>[5x]MGNNLMQTDLSVWGMYQHADIVVKCVMIGLILASVVTWAIFFSKSVEFFNQKRRLKREQQLLAEARSLNQANDIAADFGSKSLSLHLLNEAQNELELSEGSDDNEGIKERTSFRLERRVAAVGRQMGRGNGYLATIGAISPFVGLFGTVWGIMNSFIGIAQTQTTNLAVVAPGIAEALLATAIGLVAAIPAVVIYNVFARQIGGFKAMLGDVAAQVLLLQSRDLDLEASAAAHPVRVAQKLRAG;>[2x]MAMHLNENLDDNGEMHDINVTPFIDVMLVLLIIFMVAAPLATVDVKVNLPASTSTPQPRPEKPVYLSVKADNSMFIGNDPVTDETMITALNALTEGKKDTTIFFRADKTVDYETLMKVMDTLHQAGYLKIGLVGEETAKAKENLYFQGNAGSGHHHHHHHHHH

Ton is a membrane protein complex found in the inner membrane of Gram-negative bacteria. Ton can be described as a molecular motor in which the ExbB and ExbD subunits assemble to form a proton channel and use the proton gradient across the cytoplasmic membrane. The energy derived from proton translocation is propagated through the elongated TonB subunit that spans the periplasmic space and physically interacts with numerous TonB dependent transporters (TBDT) at the outer membrane, allowing the active transport of rare nutrients into the periplasm.

To gain further information on structure and stoichiometry, we performed a single particle cryo-electron microscopy (cryo-EM) analysis on the full-length ExbB–ExbD complex reconstituted in lipid nanodiscs. The final reconstruction used 85,936 particles and yielded a 3.3 Å overall resolution structure calculated without imposing symmetry. As found in the crystal structure, ExbB assembles as a pentamer, but instead of one ExbD TM domain, two TM helices of ExbD are now clearly resolved in the TM pore defined by the ExbB pentamer. The two TM helices are parallel but shifted relative to one another by half a helical turn. The two essential aspartate residues at position 25 point in opposite directions and are in close proximity to the ExbB conserved threonine residues 181 and 148 that form a ring of polar residues in the pore. The two ExbD TM helices pack tightly into the pore, with nearly 80% of surface buried for each helix, and there is no apparent channel in this configuration that would allow a proton to go through. A comparison of the EM and crystal structures shows that the most dramatic differences for ExbB are seen in shifts of some of the TM helices to accommodate the dimer of ExbD. No density is visible for the periplasmic domain of ExbD, likely because the 19-residue linker that connects the TM to the folded C-terminal domain is highly flexible. Four phospholipids were built, three PE and one PG, and are part of the cytoplasmic leaflet of the membrane. The cryo-EM experiment was performed at neutral pH (7.5), while the crystal structure that showed the single ExbD TM domain was obtained with crystals grown at acidic pH (4.5). It is likely that the cryo-EM structure represents the resting state of the Ton complex, as there is no visible channel that would connect the Asp25 residues either to the periplasm or cytoplasm.>ENLMQVYQQARLSNPELRKSAADRDAAFEKINEARSPLLPQLGLGADYTYSNGYRDANGINSNATSASLQLTQSIFDMSKWRALTLQEKAAGIQDVTYQTDQQTLILNTATAYFNVLNAIDVLSYTQAQKEAIYRQLDQTTQRFNVGLVAITDVQNARAQYDTVLANELTARNNLDNAVEQLRQITGNYYPELAALNVENFKTDKPQPVNALLKEAEKRNLSLLQARLSQDLAREQIRQAQDGHLPTLDLTASTGISDTSYSGSKTRGAAGTQYDDSNMGQNKVGLSFSLPIYQGGMVNSQVKQAQYNFVGASEQLESAHRSVVQTVRSSFNNINASISSINA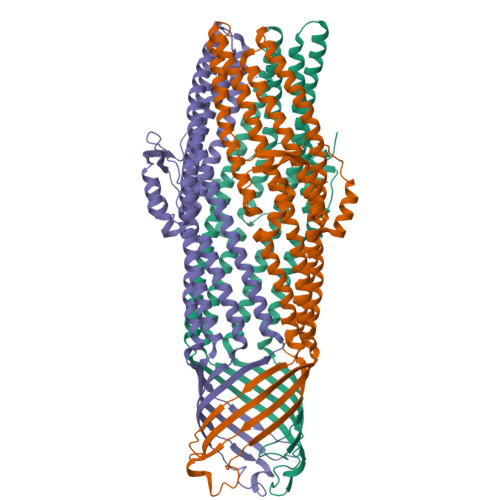YKQAVVSAQSSLDAMEAGYSVGTRTIVDVLDATTTLYNAKQELANARYNYLINQLNIKSALGTLNEQDLLALNNALSKPVSTNPENVAPQTPEQNAIADGYAPDSPAPVVQQTSARTTTSNGHNPFRN[3x]> GHMNAYLSDQPVRLSPLRDEQGNQPRFGLLLEPGRPGMHVGELPAQWLKGLARSHHLLLLRGFAAFADAESLTRYCHDFGEVMLWPFGAVLELVEQEGAEDHIFANNYVPLHWDGMYLETVPEFQVFHCVDA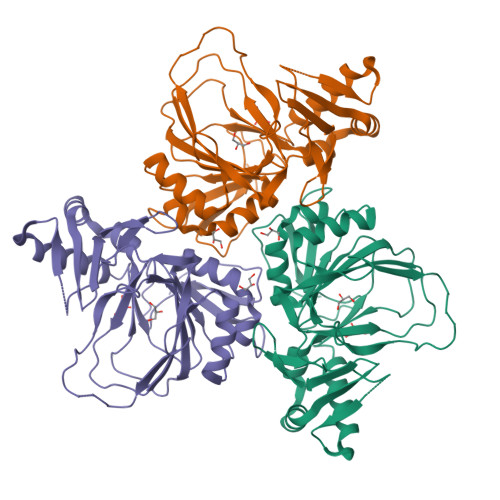PGDSDGGRTTFSSTPAALQLADSSELELWRRASGRYQRSAAHYSSRSAAPIVERHPRREFPILRFCEPPVEGDASFINPSEFHYDGIAPEQRGELLASLRRCLYHPQAHYAHRWRSDDLVIADNLTLLHGREAFAHRAPRHLRRVHIHAEPALRNPHLQRD> TADELVFFVNGKKVVEKNADPETTLLAYLRRKLGLRGTKLGCGEGGCGACTVMLSK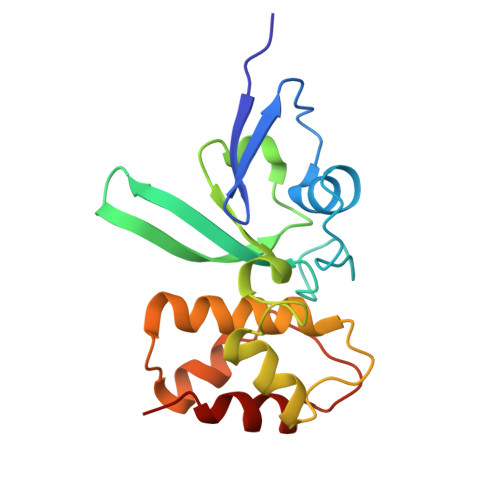YDRLQDKIIHFSANACLAPICTLHHVAVTTVEGIGSTKTRLHPVQERIAKSHGSQCGFCTPGIVMSMYTLLRNQPEPTVEEIEDAFQGNLCRCTGYRPILQGFRTFAK>GASKLRAVLEKLKLSRDDISTAAGMVKGVVDHLLLRLKCDSAFRGVGLLNTGSYYEHVKISAPNEFDVMFKLEVPRIQLEEYSNTRA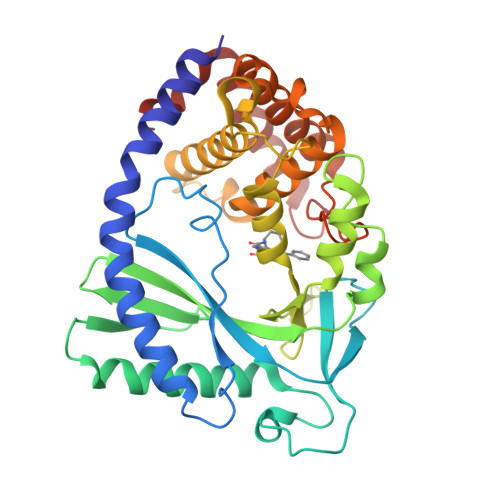YYFVKFKRNPKENPLSQFLEGEILSASKMLSKFRKIIKEEINDIKDTDVIMKRKRGGSPAVTLLISEKISVDITLALESKSSWPASTQEGLRIQNWLSAKVRKQLRLKPFYLVPKHAKEGNGFQEETWRLSFSHIEKEILNNHGKSKTCCENKEEKCCRKDCLKLMKYLLEQLKERFKDKKHLDKFSSYHVKTAFFHVCTQNPQDSQWDRKDLGLCFDNCVTYFLQCLRTEKLENYFIPEFNLFSSNLIDKRSKEFLTKQIEYERNNEFPVFDEF[2x]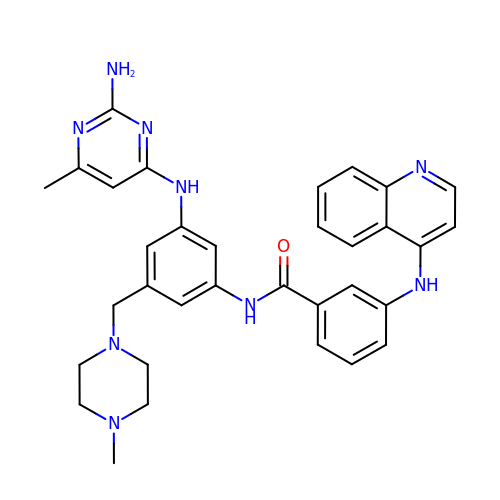N-{3-[(2-amino-6-methylpyrimidin-4-yl)amino]-5-[(4-methylpiperazin-1-yl)methyl]phenyl}-3-[(quinolin-4-yl)amino]benzamide | C33 H35 N9 O | HSJHGRCPBQHRPX-UHFFFAOYSA-N>[2x]MRCIGISNRDFVEGVSGGSWVDIVLEHGSCVTTMAKNKPTLDFELIETEAKQPATLRKYCIEAKLTNTTTDSRCPTQGEPSLNEEQDKRFVCKHSMVDRGWGNGCGLFGKGGIVTCAMFT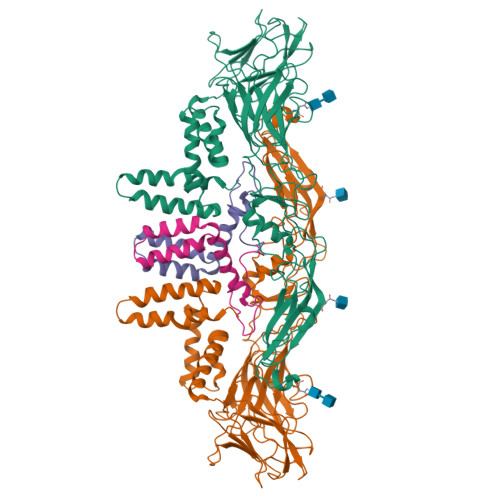CKKNMKGKVVQPENLEYTIVITPHSGEEHAVGNDTGKHGKEIKITPQSSITEAELTGYGTVTMECSPRTGLDFNEMVLLQMENKAWLVHRQWFLDLPLPWLPGADTQGSNWIQKETLVTFKNPHAKKQDVVVLGSQEGAMHTALTGATEIQMSSGNLLFTGHLKCRLRMDKLQLKGMSYSMCTGKFKVVKEIAETQHGTIVIRVQYEGDGSPCKIPFEIMDLEKRHVLGRLITVNPIVTEKDSPVNIEAEPPFGDSYIIIGVEPGQLKLNWFKKGSSIGQMIETTMRGAKRMAILGDTAWDFGSLGGVFTSIGKALHQVFGAIYGAAFSGVSWIMKILIGVIITWIGMNSRSTSLSVSLVLVGVVTLYLGVMVQA;>[2x]SVALVPHVGMGLETATETWMSSEGAWKHAQRIETWILRHPGFTIMAAILAYTIGTTHFQRALIFILLTAVAPSMT In the best-characterized E3-E3 pathways, ARIH-family RING-between-RING (RBR) E3s ligate ubiquitin to substrates of neddylated cullin-RING E3s. The E3 ARIH2 has been implicated in ubiquitylation of substrates of neddylated CUL5-RBX2-based E3s, including APOBEC3-family substrates of the host E3 hijacked by HIV-1 virion infectivity factor (Vif). Structures of ARIH2 alone and bound to neddylated CRL5Vif-CBFβ reveal the HIV-1 hijacked E3-E3 ligase assembly that overcomes host restriction and defines mechanisms by which NEDD8-linked CUL5-RBX2 activates ARIH2.

The two ARIH2 molecules in the asymmetric unit superimpose with 0.6 Å root mean square deviation (r.m.s.d.), hence only one is described. The canonical RBR E3 catalytic elements (RING1, RTI helix, in-between RING (IBR) and Rcat domains) are interspersed with the ARIH-specific UBA-like (UBAL) and Ariadne domains in a two-part arrangement. The ARIH2 UBAL, RING1, RTI helix and IBR domains form an E2~UB-binding platform. The arrangement of the RING1, RTI helix and IBR domains in autoinhibited ARIH2 resembles that in activated ARIH1 bound to UBE2L3~UB. ARIH2’s UBAL domain stabilizes the E2~UB-binding platform on the opposite side, by intercalating between the RING1 and IBR domains, and packing against the RTI helix.Fig. 1 a, ARIH2 schematic color-coded by domains. The second part of the ARIH2 structure shows autoinhibition: the Ariadne domain binds the active site in the catalytic Rcat domain. The Ariadne domain is an elongated four-helix bundle. A groove between the first and third helices of the Ariadne domain secures the catalytic cysteine loop from the Rcat domain. In particular, Ariadne domain residues Leu381, Glu382 and Glu455, respectively, contact the beginning, middle and end of the Rcat domain catalytic cysteine loop. The second crucial portion of ARIH2 is its N-terminal region, which is not present in the crystal structure.

>[2x]MSVDMNSQGSDSNEEDYDPNCEEEEEEEEDDPGDIEDYYVGVASDVEQQGADAFDPEEYQFTCLTYKESEGALNEHMTSLASVLKVSHSVAKLILVNFHWQVSEILDRYKSNSAQLLVEARVQPNPSKHVPTSHPPHHCAVCMQFVRKENLLSLACQHQFCRSCWEQHCSVLVKDGVGVGVSCMAQDCPLRTPEDFVFPLLPNEELREKYRRYLFRDYVESHYQLQLCPGADCPMVIRVQEPRARRVQCNRCNEVFCFKCRQMYHAPTDCATIRKWLTKCADDSETANYISAHTKDCPKCNICIEKNGGCNHMQCSKCKHDFCWMCLGDWKTHGSEYYECSRYKENPDIVNQSQQAQAREALKKYLFYFERWENHNKSLQLEAQTYQRIHEKIQERVMNNLGTWIDWQYLQNAAKLLAKCRYTLQYTYPYAYYMESGPRKKLFEYQQAQLEAEIENLSWKVERADSYDRGDLENQMHIAEQRRRTLLKDFHDT Cryptic unstable transcripts (CUTs) are rapidly degraded by the nuclear exosome in a process requiring the RNA helicase Mtr4 and specific adaptor complexes for RNA substrate recognition. The eleven-subunit MTREC comprises the zinc-finger protein Red1 and the Mtr4 homologue Mtl1. The zinc-finger protein Red1 serves as the main scaffold for the entire MTREC complex, assembling the individual submodules, including the Mtl1 helicase, into a large complex. Therefore, Red1 essentially acts as an adaptor between Mtl1 and the various MTREC submodules to provide a route for RNA substrates to the exosome through the unwinding activity of Mtl1.

We therefore decided to explore different strategies, including generating a single-chain construct in which ctRed1pep is fused to the C-terminus of ctMtr4SA via a short linker (ctMtr4SA–ctRed1pep construct). The single-chain ctMtr4SA–ctRed1pep complex was readily crystallized and the crystals diffracted to 1.99 Å resolution. The structure was determined de novo using the anomalous signal of the bound Zn2+ (Zn-SAD), whose identity was confirmed by X-ray fluorescence (XRF) emission spectrum analysis. The asymmetric unit (ASU) contains two molecules of the single-chain complex, which exhibit very small differences as indicated by the low root-mean-square deviation (RMSD) of 1.02 Å for Cα atoms of 269 residues. The ctMtr4 short arch superimposed well with the scMtr4 structure, revealing that the ctRed1 peptide is positioned on top of the KOW domain. The N-terminal region (residues 1017–1024) of the peptide contains several highly conserved residues, among them Tyr1017 and Ser1019, which form hydrogen bonds with Glu854 from the stalk. Furthermore, Pro1020, Leu1021, and Phe1024 of ctRed1pep pack against Ile668, Met675, Met679, Leu847, and Ile850 of the stalk helices. These interactions are followed by a U-shaped structure (residues 1025–1046), which is positioned between the stalk-interacting and the KOW-interacting residues of the peptide. Residues 1047–1080 exclusively interact with the KOW domain, including more hydrophobic interactions mediated by Ile1050, Met1056, Leu1061, Phe1075, and Ile1078, which pack against Ile790, Leu792, Val819, Phe823, and Pro828. The middle part of the peptide (residues 1047–1056) is stabilized and held in position by the conserved Zn-finger of ctRed1, composed of Cys1057, Cys1066, Cys1070, and His1074 (inset).

>MDEALIKDYHSIREQIDQYTKDMVLVMQHPTNCVKYINPGRLMHVVTSDGTDFGWGVIINFYERRPERNNPNPGWSPQESYVVEVLLRLSSDSGSVDSKLKDNQCIPAGIAPVTQKNDPGRWEVVPCLLSCMHGLSQIKLHVPDKKSGGSMDDPETRRRVGKSLLEVQRRFEDGIPHMDPIENMHIRDVEFKKLLRKIEVLESRLVANPLHNSGGSGGS[2x];>[2x]ALSYSSPLRFFRNFRFHPEFTRLVAGGWRSLTYSSRIDPDKEMCPYELEGTQCPSGCSFQHFVDITPAADERILLELSGSHHHHHH>GCGVEEKTEVQLLKEMPKPKAMTIDPSLSQKEATEMVHAAQRFYAFWDTGKEELIPQTVTENFFDHTLPKGRPQGTEGLKFAAQNFRKIVPNIHCEIEDLLVVGDKVTARLSFTGTHNDKKIDFFAIDILHVKDGKITEDWHLEDNLTLKQQLGLI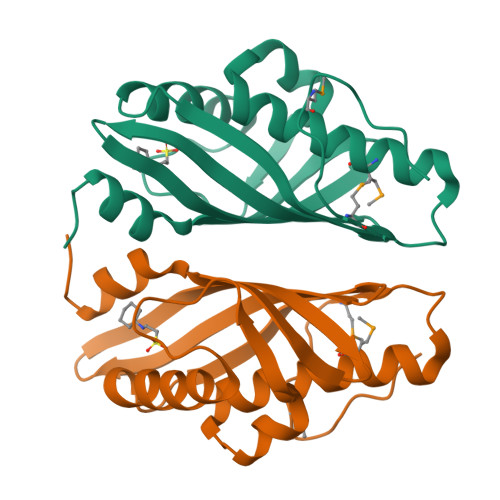AEE[2x]>GAEIPKEMLRAQTNXILLNVLKQGDNYVYGIIKQVKEASNGEMELNEATLYTIFDRLEQDGIISSYWGDESQGGRRKYYRLTEIGHENMRLAFE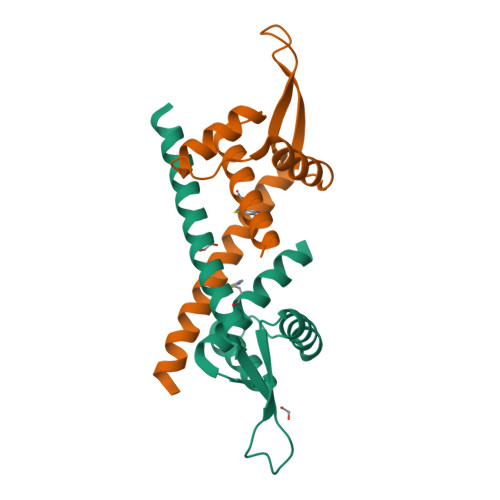SWSRVDKIIENLEANKKSEAIKSRGGSGGWSHPQFEK[2x]>[4x]MASRGVNKVILVGNLGQDPEVRYMPNGGAVANITLATSESWRDKATGEMKEQTEWHRVVLFGKLAEVASEYLRKG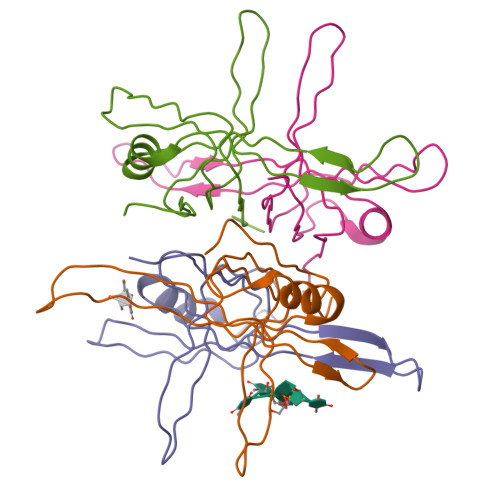SQVYIEGQLRTRKWTDQSGQDRYTTEVVVNVGGTMQMLGGRQGGGAPAGGNIGGGQPQGGWGQPQQPQGGNQFSGGAQSRPQQSAPAAPSNEPPMDFDDDIPF> EKLYGIPHNGFWNQRRMYTEARGQTAALAAMQDPVEVLNFAGSNEMASTYLLVSCLRRVSALCDKKHAVLETVAKDERLQRLIQLISPHVDDCDARCLVDLCWAVWGFRGAPDVVEPLLNRMASVVVRRENAFTPKQLGTIAFTFSWFRGAPTDTVADFVLAECVKLLPEMEPFHVTLLFGSLRRMRRLNRDVANLMIEKLTDDIDRFTSDDVVGVLRALAANSITRGFLLRRVATLVFDNLDSFKPKQLASVLNSLTLLRFLTVENGEELFSCLSGSLSELPAASIAEILEALTILNFPRPEVVRTCLDLLAEKNGLISQGSWVRDHMIIAAHAVIQFQLYDKNPVVKPLLEELFRSRVN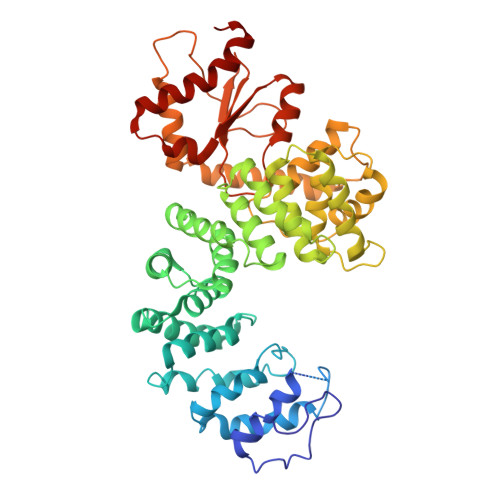SSRTQHRVEEVIHALDLEKASPRVDVPPYWRAMIDQANREEQARLEHSGLQNELTLVLDSLRGKFQLQIQKNQQAGPYSVQFLDDETKICIEIDYPCCRTPHIIKARHLKQLGYHYLLVDCWQWRRLRSEAEQTVFLKQLLSGPLLEVGRL> MKKGGLLLILLILVSIASGCISESNENQTATASTVPPTSVTPSQSSTPTTSTSTYGPSERTELKLPSVNYT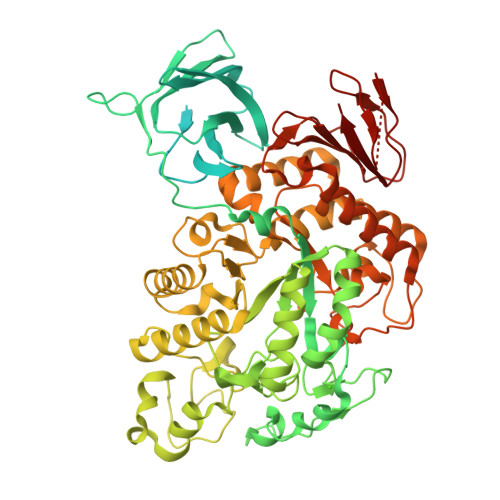PIYVGIEKGCPSGRVPVKFTYNPGNKTVKSVSLRGSFNNWGEWPMELKNGTWETTVCLRPGRYEYKYFINGQWVKDMSDDGTGRPYDPDADAYAPDGYGGKNAVRVVEGREAFYVEFDPRDPAYLSIADKRTVVRFEAKRDTVESAVLVTDHGNYTMKLQVWWDFGETWRAEMPVEPADYYILVTSSDGGKFAVLNTSESPFFHFDGVEGFPQLEWVSNGITYQIFPDRFNNGNKSNDALALDHDELILNQVNPGQPILSNWSDPITPLHCCHQYFGGDIKGITEKLDYLQSLGVTIIYINPIFLSGSAHGYDTYDYYRLDPKFGTEDELREFLDEAHRRGMRVIFDFVPNHCGIGNPAFLDVWEKGNESPYWDWFFVKKWPFKLGDGSAYVGWWGFGSLPKLNTANQEVREYLIGAALHWIEFGFDGIRVDVPNEVLDPGTFFPELRKAVKEKKPDAYLVGEIWTLSPEWVKGDRFDSLMNYALGRDILLNYAKGLLSGESAMKMMGRYYASYGENVVAMGFNLVDSHDTSRVLTDLGGGKLGDTPSNESIQRLKLLSTLLYALPGTPVTFQGDERGLLGDKGHYDEQRYPIQWDTVNEDVLNHYRALAELRKRVPALRSSAMRFYTAKGGVMAFFRGHHDEVLVVANSWKKPALLELPEGEWKVIWPEDFSPELLRGTVEVPAIGIIILERG GERANYLGERANYL DIPHOSPHATE | C20 H36 O7 P2 | 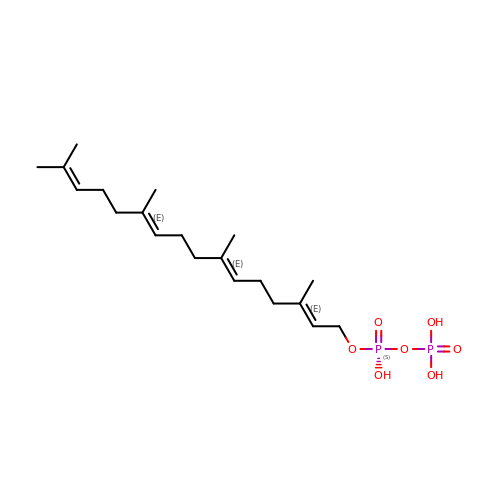OINNEUNVOZHBOX-QIRCYJPOSA-N> MVPISPIETVPVKLKPGMDGPKVKQWPLTEEKIKALVEICTEMEKEGKISKIGPENPYNTPVFAIKKKDSTKWRKLVDFRELNKRTQDFWEVQLGIPHPAGLKKKKSVTVLDVGDAYFSVPLDEDFRKYTAFTIPSINNETPGIRYQYNVLPQGWKGSPAIFQSSMTKILEPFKKQNPDIVIYQYMDDLYVGSDLEIGQHRTKIEELRQHLLRWGLTTPDKKHQKEPPFLWMGYELHPDKWTVQPIVLPEKDSWTVNDIQKLVGKLNWASQIYPGIKVRQLSKLLRGTKALTEVIPLTEEAELELAENREILKEPVHGVYYDPSKDLIAEIQKQGQGQWTYQIYQEPFKNLKTGKYARMRGAHTNDVKQLTEAVQKITTESIVIWGKTPKFKLPIQKETWETWWTEYWQATWIPEWEFVNTPPLVKLWYQLEKEPIVGAETFYVDGAANRETKLGKAGYVTNKGRQKVVPLTNTTNQKTELQAIYLALQDSGLEVNIVTNSQYA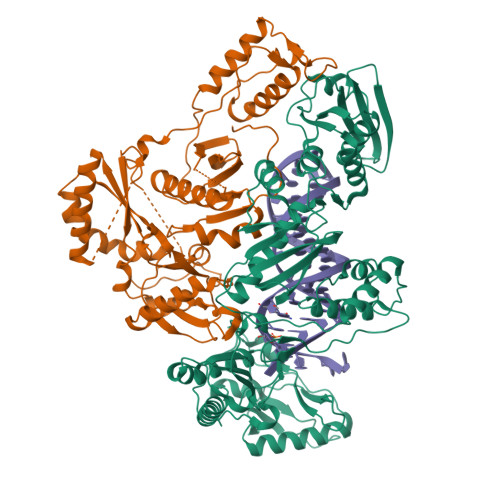LGIIQAQPDKSESELVNQIIEQLIKKEKVYLAWVPAHKGIGGNEQVDKLVSAG;> MAHHHHHHALEVLFQGPISPIETVPVKLKPGMDGPKVKQWPLTEEKIKALVEICTEMEKEGKISKIGPENPYNTPVFAIKKKDSTKWRKLVDFRELNKRTQDFWEVQLGIPHPAGLKKKKSVTVLDVGDAYFSVPLDEDFRKYTAFTIPSINNETPGIRYQYNVLPQGWKGSPAIFQSSMTKILEPFKKQNPDIVIYQYMDDLYVGSDLEIGQHRTKIEELRQHLLRWGLTTPDKKHQKEPPFLWMGYELHPDKWTVQPIVLPEKDSWTVNDIQKLVGKLNWASQIYPGIKVRQLCKLLRGTKALTEVIPLTEEAELELAENREILKEPVHGVYYDPSKDLIAEIQKQGQGQWTYQIYQEPFKNLKTGKYARMRGAHTNDVKQLTEAVQKITTESIVIWGKTPKFKLPIQKETWETWWTEYWQATWIPEWEFVNTPPLVKLWYQ> QDSRGCARWCPQNSSCVNATACRCNPGFSSFSEIITTPTETCDDINECATPSKVSCGKFSDCWNTEGSYDCVCSPGYEPVSGAKTFKNESENTCQDVDECSSGQHQCDSSTVCFNTVGSYSCRCRPGWKPRHGIPNNQKDTVCED;> SDCGLPPDVPNAQPALEGRTSFPEDTVITYKCEESFVKIPGEKDSVICLKGSQWSDIEEFCNRSCEVPTRLNSASLKQPYITQNYFPVGTVVEYECRPGYRREPSLSPKLTCLQNLKWSTAVEFCKKKSCPNPGEIRNGQIDVPGGILFGATISFSCNTGYKLFGSTSSFCLISGSSVQWSDPLPECREIYCPAPPQIDNGIIQGERDHYGYRQSVTYACNKGFTMIGEHSIYCTVNNDE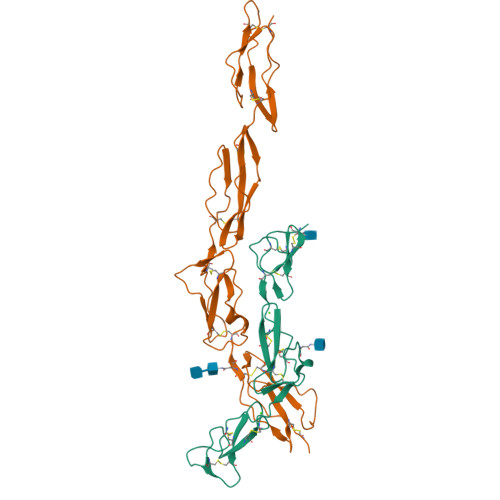GEWSGPPPECR>TASPSALADELEQLAYEVEHLSS[4x];>[4x]TASPHALANRLRQLAYRVRSLS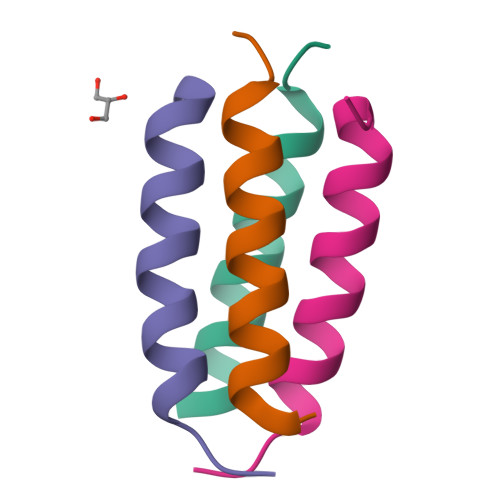S> MAHHHHHHAREPISLDQTIGDEGDSQLGDFIEDSEAVVAVDAVSFTLLQDQLQSVLDTLSEREAGVVRLRFGLT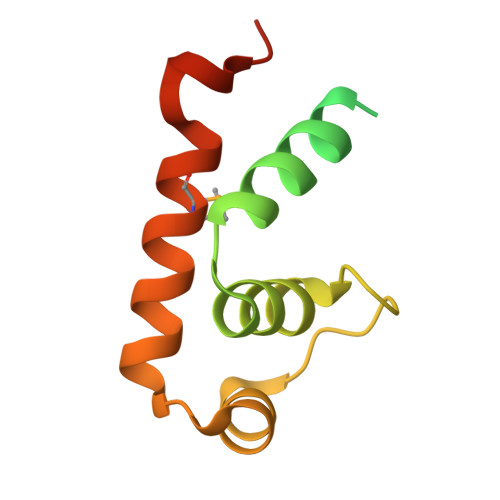DGQPRTLDEIGQVYGVTRERIRQIESKTMSKLRHPSRSQVLRDYLD>MTARPENPSTVHDFVGIGLGPFNLGLACLTEPIDELDGIFLESKPDFEWHAGMFLDGAHLQTPFMSDLVTLADPTSPYSFLNYLKEKGRLYSFYIRENFYPLRVEYDDYCRWAANKLSSIRFGTTVTEVRYEDDLYVVTTSAGDVYRARHLVLGTGTPPYIPEACQGLDGDFIHNSRYVQHRSELVKKESITIVGSGQSAAEIYQDLLGEIDVHGYRLNWVTRSPRFFPLEYTKLTLEMTSPEYIDYYRELPEATRYRLTAEQKGLFKGIDGDLINEIFDLLYQKNLAGPVPTRLLTNS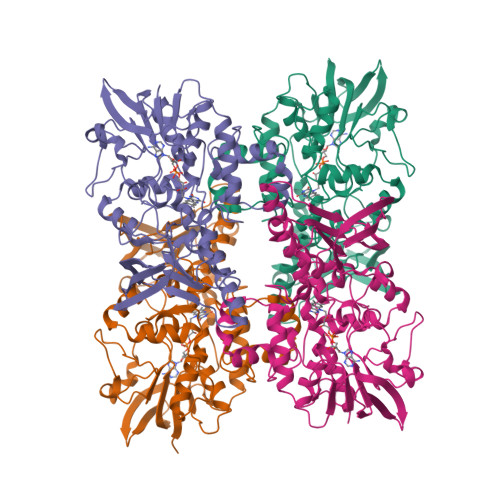SLNSARHENGTYTLAFRQEEQGKDFEIESQGLVLATGYKYAEPEFLAPVKDRLVYDSQGNFDVSRAYAIDVTGRGVFLQNAGVHTHSITSPDLGMGAYRNSCIIRELLGTEYYPVEKTIAFQEFSV[8x]> MSRLFVKRLPTGSFLMLLLYIGLLLSAIAVAYSTYWNRQLLNSLYSELSVRDKAQAEWGRLILEQSTWTAHSRIESLAVEQLRMRVPDPAEV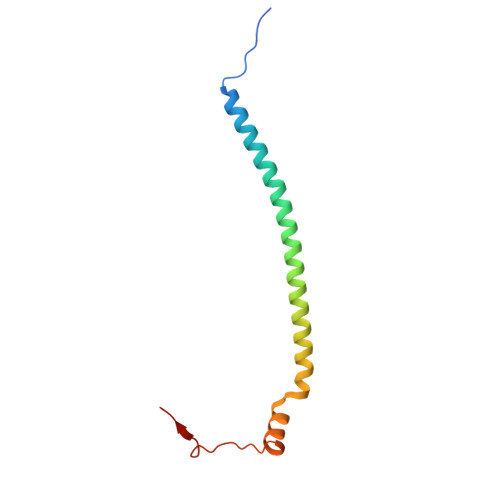RMVAP2-(pyridin-3-yl)benzoic acid | C12 H9 N O2 | 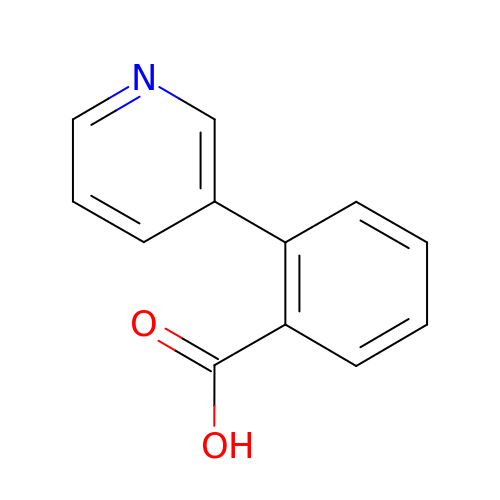DRGNPLUCFXKUAL-UHFFFAOYSA-N>GSESQVLRGTGHCKWFNVRMGFGFISMINREGSPLDIPVDVFVHQSKLFMEGFRSLKEGEPVEFTFKKSS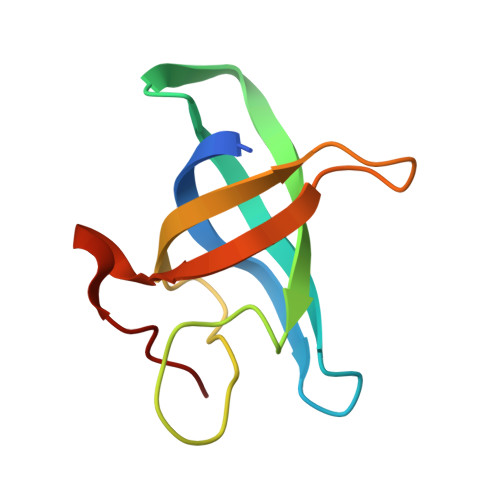KGLESIRVTGPGGSPCLGSE[2x]> 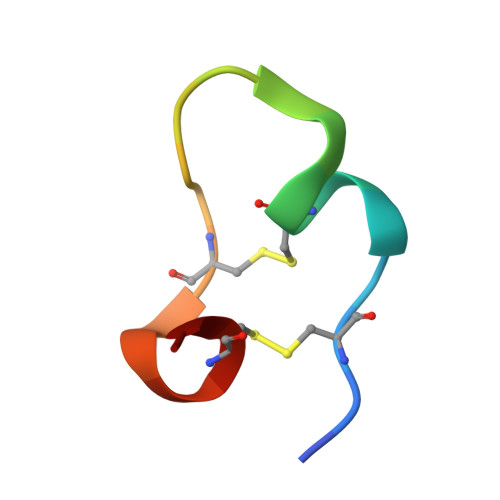VQCPHFCYELDYELCPDVCYV> KYNMGNANYRIQKELHNFLNNPPINCTLDVHPNNIR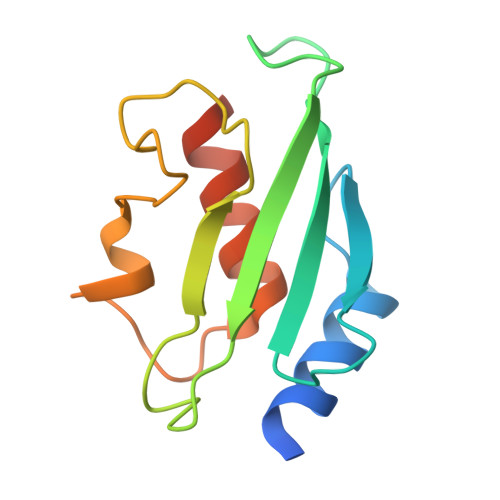IWIVKYVGLENTIYANEVYKLKIIFPDDYPLKPPIVYFLQKPPKHTHVYSNGDICLSLLGDDYNPSLSISGLVLSIISMLSSAKEKKLP> QFAKPEDAVKYRQSAFTLMASHFGRMTPVVKGQAPYDAAQIKANVEVLKTLSALPWAAFGPGTEGGDARPEIWSDAASFKQKQQAFQDNIVKLSAAADAGDLDKLRAAFGDVGASCKACHDAYRKK

Cytochromes c′ occur in methanotrophic, denitrifying and photosynthetic bacteria and have proposed roles in protection against nitrosative stress, NO trafficking during denitrification or pathogen defence. All cytochromes c′ have a 4 α-helix bundle structure containing a heme centre with a solvent exposed proximal His ligand and a buried hydrophobic distal pocket with a non-coordinated residue (Leu or Phe, rarely Met or Tyr) in a position to exert steric influence on the binding of diatomic gases. Unusually, cytochromes c′ are able to utilize both heme faces (distal and proximal) as a means of discriminating NO from other diatomic gases. In order to understand the factors controlling distal versus proximal NO coordination, we have examined NO binding to AXCP variants in which the occluding distal residue Leu16 is replaced with residues that are smaller (Ala, Val), of comparable size (Ile) or larger (Phe).

All of the tertiary structures are similar to wt AXCP and only salient points concerning the heme region are discussed here.(3~{R})-2-[(5-chloranylpyridin-2-yl)methyl]-3-(4-chlorophenyl)-4-fluoranyl-3-[(1-oxidanylcyclopropyl)methoxy]-6-(2-oxidanylpropan-2-yl)isoindol-1-one 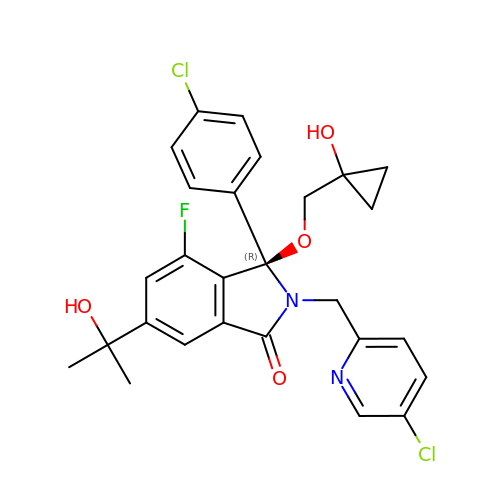| C27 H25 Cl2 F N2 O4 | LAGWUKAFTJACQB-HHHXNRCGSA-N>EDICFIAGIGDTNGYGWGIAKELSKRNVKIIFGIWPPVYNIFMKNYKNGKFDNDMIIDKDKKMNILDMLPFDASFDTANDIDEETKNNKRYNMLQNYTIEDVANLIHQKYGKINMLVHSLANAKEVQKDLLNTSRKGYLDALSKSSYSLISLCKYFVNIMKPQSSIISLTYHASQKVVPGYGGGMSSAKAALESDTRVLAYHLGRNYNIRINTISAGPLKSRAATAINK[2x];>YTFIDYAIEYSEKYAPLRQKL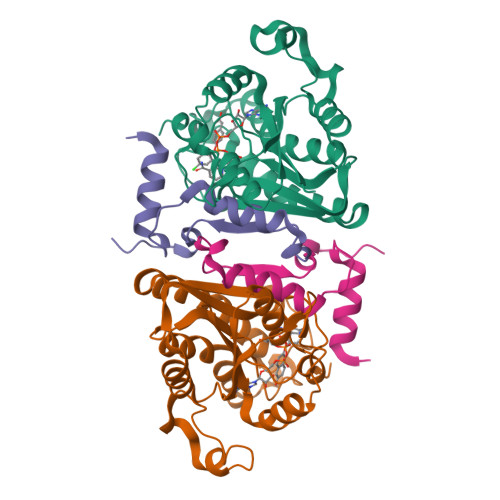LSTDIGSVASFLLSRESRAITGQTIYVDNGLNIMFLPDD[2x]> MLSVAARSGPFAPYLSAAAHAVPG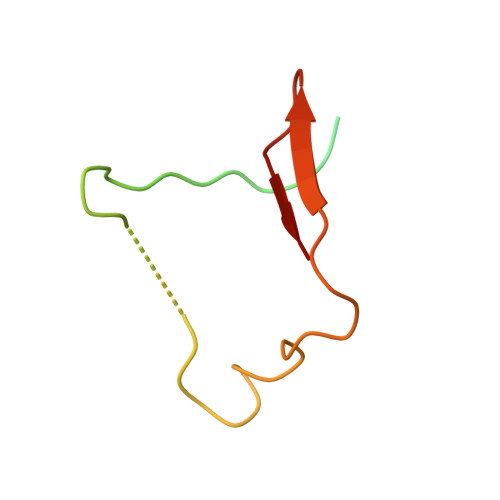PLKAXXXXXXXXXXXXXXLKRPLLCRESMSGRSARRDLVAGISLNAPASVRY>[6x]M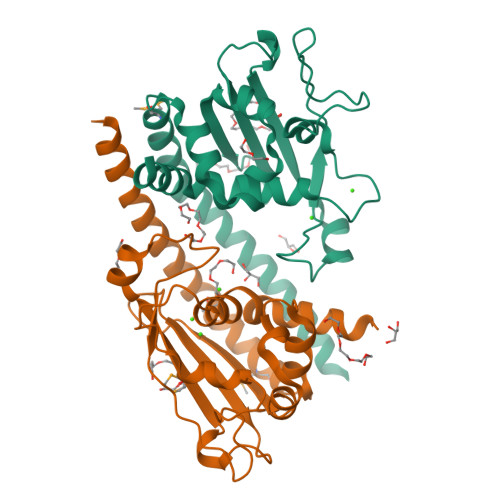SAKKTNEKRSEIQSETNTTSLDEVADIELEFEKADVELLKHQVELFNPLYEKRAMVLRKIPKFWPIAIEAAPSDELSVYISPEDANVLEHLIDLRVYRPNEDPRDIKIVFEFEANEYLESNSLYLMKLFRYSSQKAEASSSNINKEPSQLISEKVNIEWKKNKDLTRQTKGTAPSFFTWFSWTGKENDIFEDEEELAIFIAEDLYPNAVKYFTDALQENEENEDEEIDLENENGDNISEEEPSKKRTKL>GHMGVDGLLEDKALVEAALFVAGRPLSLKELSKALGIKSLEYLEKLIELIASEYEERKSAIEVVKVLGDKWVMQLKQEYSQKVIHLMPKPELRAGELKTLALIAYLQPVEQSKIIKLRGSQAYEHIKKLLEMGLIYAEPYERTKLLGTTQKFAELYGFPENDPELIKEAF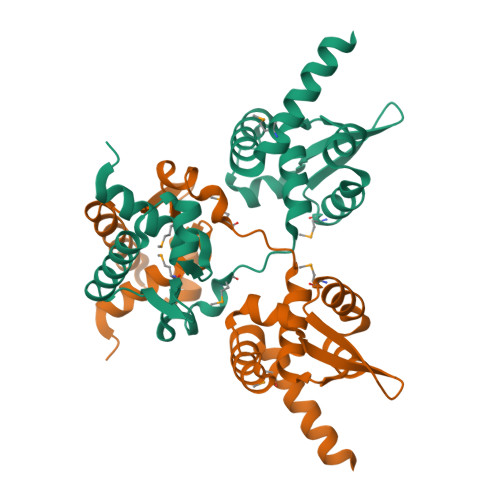KKVIHSEYADLMEKIEKNNRKDKREEA[2x]> GAMDPEFMELRVGNRYRLGRKIGSGSFGDIYLGTDIAAGEEVAIKLECVKTKHPQLHIESKIYKMMQGGVGIPTIRWCGAEGDYNVMVMELLGPSLEDLFNFCSRKFSLKTVLLLADQMISRIEYIHSKNFIHRDVKPDNFLMGLGKKGNLVYIIDFGLAKKYRDARTHQHIPYRENKNLTGTARYASINTHLGIEQSRRDDLESLG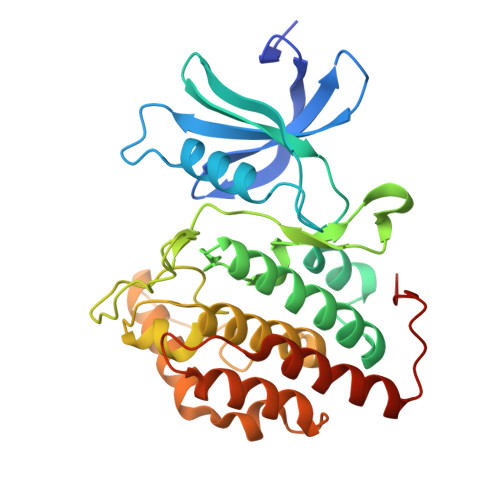YVLMYFNLGSLPWQGLKAATKRQKYERISEKKMSTPIEVLCKGYPSEFATYLNFCRSLRFDDKPDYSYLRQLFRNLFHRQGFSYDYVFDWNMLK The importance of the ubiquitin ligase murine double mutant 2 (MDM2) as a key negative regulator of the tumour suppressor protein p53 has been studied extensively. Second, it promotes the proteasomal degradation of p53 by recruiting Ub conjugating enzyme (E2) thioesterified with ubiquitin (E2~Ub; ~ indicates thioester bond) via its RING domain and mediates ubiquitin (Ub) transfer from E2 to p53,8 where Ub is preferentially conjugated to lysine residues located in the C-terminal lysine rich region of p53.9 Although the relative importance of these mechanisms is context dependent, in vivo mouse studies with ligase defective MDM2 resulted in the same lethality as MDM2 knockout experiments. The RING domain of MDM2 has been discussed as an alternative target to stabilize p53.19 The rationale for this approach lies in MDM2′s ability to still bind and inhibit p53 when MDM2-mediated ubiquitination is abolished, thereby preventing uncontrolled activation of p53.8 The RING domain gains its E3 ligase activity through dimerization with either itself or the RING domain of its catalytic inactive homologue MDMX to form a homodimer or heterodimer, respectively. The dimeric RING domain arrangement is essential for E2~Ub binding and activation as demonstrated by co-crystal structures with UbcH5B–Ub (en dash indicates covalent complex).

We wondered whether the sequence dissimilarity induced structural differences that could account for the different aggregation tendencies of the MDM2 variants and performed protein crystallization for MDM2f and MDM2z. Likewise, the asymmetric unit of the MDM2f crystal contains two molecules of MDM2f, which form a dimer. Similar to MDM2z, there was no electron density for residues located N-terminal to the RING domain (414–424, corresponding to 423–433 in MDM2h). The major difference is the absence of electron density for the 310-helix preceding the RING domain. A possible explanation for this observation could be the sequence difference for residues preceding the RING domain, which form a 310-helix in MDM2h but lack electron density in all MDM2f and MDM2z structures reported in this study. The helices are stabilized by a tight hydrophobic packing arrangement involving residues A434 and F490 of each protomer. In MDM2f and MDM2z, A434 is replaced with serine and cysteine, respectively. Both serine and cysteine would likely cause a steric clash and their polar side chains would disrupt the hydrophobic packing, thereby precluding a similar helical arrangement.

>[2x]GSDESMEPSLPLTSVEPCVICQTRPKNGCIVHGRTGHLMACYTCAKKLKKRNKPCPVCREPIQMIVLTYFS> ESTVTEELKEGIDAVYPSLVGTADSKAEGIKNYFKLSFTL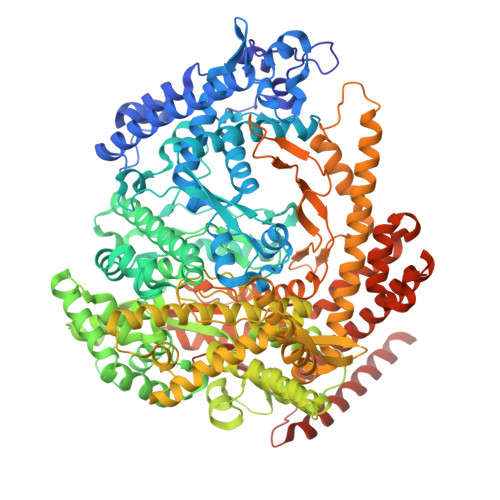PEEQKSRTVGSEAPLKDVAQALSSRARYELFTEKETANPAFNGEVIKRYKELMEHGEGIADILRSRLAKFLNTKDVGKRFAQGTEANRWVGGKLLNIVEQDGDTFKYNEQLLQTAVLAGLQWRLTATSNTAIKDAKDVAAITGIDQALLPEGLVEQFDTGMTLTEAVSSLAQKIESYWGLSRNPNAPLGYTKGIPTAMAAEILAAFVESTDVVENIVDMSEIDPDNKKTIGLYTITELDSFDPINSFPTAIEEAVLVNPTEKMFFGDDIPPVANTQLRNPAVRNTPEQKAALKAEQATEFYVHTPMVQFYETLGKDRILELMGAGTLNKELLNDNHAKSLEGKNRSVEDSYNQLFSVIEQVRAQSEDISTVPIHYAYNMTRVGRMQMLGKYNPQSAKLVREAILPTKATLDLSNQNNEDFSAFQLGLAQALDIKVHTMTREVMSDELTKLLEGNLKPAIDMMVEFNTTGSLPENAVDVLNTALGDRKSFVALMALMEYSRYLVAEDKSAFVTPLYVEADGVTNGPINAMMLMTGGLFTPDWIRNIAKGGLFIGSPNKTMNEHRSTADNNDLYQASTNALMESLGKLRSNYASNMPIQSQIDSLLSLMDLFLPDINLGENGALELKRGIAKNPLTITIYGSGARGIAGKLVSSVTDAIYERMSDVLKARAKDPNISAAMAMFGKQAASEAHAEELLARFLKDMETLTSTVPVKRKGVLELQSTGTGAKGKINPKTYTIKGEQLKALQENMLHFFVEPLRNGITQTVGESLVYSTEQLQKATQIQSVVLEDMFKQRVQEKLAEKAKDPTWKKGDFLTQKELNDIQASLNNLAPMIETGSQTFYIAGSENAEVANQVLATNLDDRMRVPMSIYAPAQAGVAGIPFMTIGTGDGMMMQTLSTMKGAPKNTLKIFDGMNIGLNDITDASRKANEAVYTSWQGNPIKNVYESYAKFMKNVDFSKLSPEALEAIGKSALEYDQRENATVDDIANAASLIERNLRNIALGVDIRHKVLDKVNLSIDQMAAVGAPYQNNGKIDLSNMTPEQQADELNKLFREELEARKQKVAK> MKHQHQHQHQHQHQQPLQEEEQAHATSLPPRASSPPQILPQLSPEQLGMIEKLVAAQQQCNRRSFSDRLRVTPWPMAPDPHSREARQQRFAHFTELAIVSVQEIVDFAKQLPGFLQLSREDQIALLKTSAIEVMLLETSRRYNPGSESITFLKDFSYNREDFAKAGLQVEFINPIF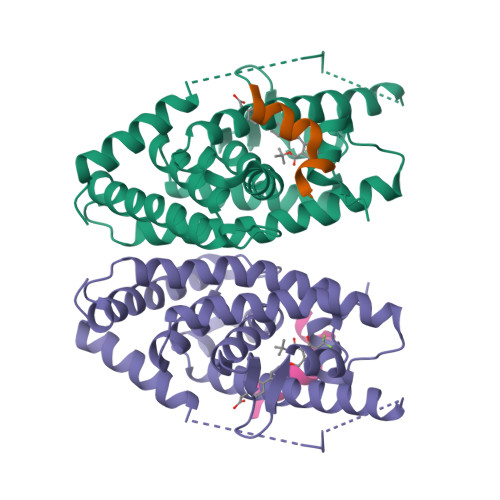EFSRAMNELQLNDAEFALLIAISIFSADRPNVQDQLQVERLQHTYVEALHAYVSIHHPHDRLMFPRMLMKLVSLRTLSSVHSEQVFALRLQDKKLPPLLSEIWDVHE;> CPSSHSSLTERHKILHRLLQEGSPS> MHHHHHHSSGRENLYFQGHMETSVPPGSALVGPSCVMDDFRDPQRWKECAKQGKMPCYFDLIEENVYLTERKKNKSHRDIKRMQCE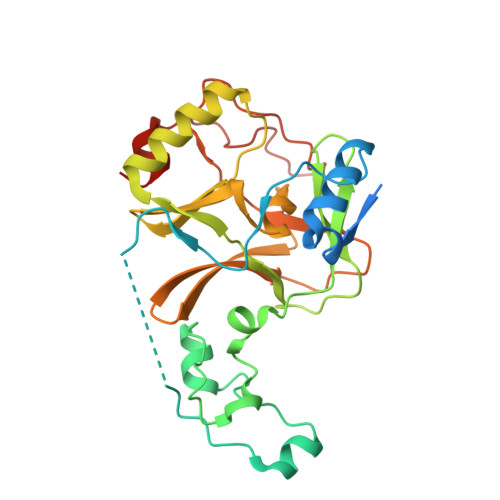CTPLSKDERAQGEIACGEDCLNRLLMIECSSRCPNGDYCSNRRFQRKQHADVEVILTEKKGWGLRAAKDLPSNTFVLEYCGEVLDHKEFKARVKEYARNKNIHYYFMALKNDEIIDATQKGNCSRFMNHSCEPNCETQKWTVNGQLRVGFFTTKLVPSGSELTFDYQFQRYGKEAQKCFCGSANCRGYLGGENRVSIRAAGGKMKKERSRK>[2x]AT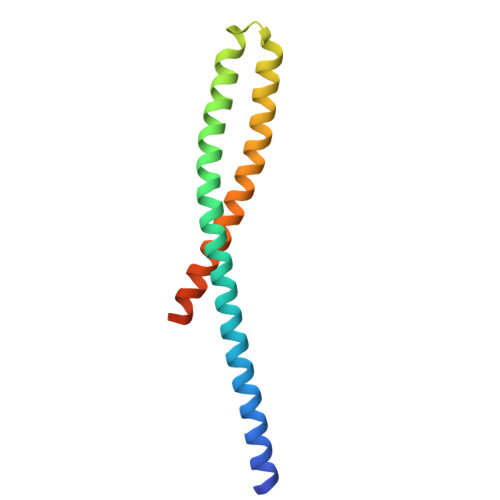DAASLVGELQALDAEYQNLANQEEARFNEERAQADAARQALAQNEQVYNELSQRAQRLQAEANTRFYKSQYQEAASKYEDALKKLEAEMEQQKAVISDFEKIQALRAGNLEHHHHHH M1 from influenza C virus (M1-C) has been shown to be the key component in inducing the formation of protrusions, called cord-like structures (CLS), emanating out of infected cells and in regulating their growth thus demonstrating a role for M1-C in membrane remodeling. We show that the N-terminal domain of M1-C adopts a similar fold as M1-A, despite the low sequence homology of both proteins, but coordinates two Mg2+ ions which increases the positive surface charge and may thus facilitate electrostatic interactions with negatively charged membranes. Full length M1-C adopts an elongated structure that tends to polymerize into ring-like or filamentous structures via lateral interactions of M1-C protomers. Our study thus confirms that M1-C assembly on membranes constitutes the driving force for influenza C virus bud formation.

We solved the crystal structure of C-terminally truncated M1-C, (NTD, residues 1–155) by single anomalous dispersion (SAD) techniques to a resolution of 1.5 Å. The structure is composed of a tandem repeat of two four-helical bundles (helices 1–4 and 6–9) that are connected by a long linker containing helix 5. Interactions between the two four helical bundles and with the linker are hydrophobic as in the case of M1-A structures28293139. The overall fold is similar to known M1-A NTD crystal structures28293139, albeit their low sequence homology. Major changes are observed for the position of helix 6, which moves approximately 10 Å outwards. A notable difference between the M1-A and M1-C structures is the unexpected coordination of 2 Mg2+ ions by helix 5 residues. The first Mg2+ ion is coordinated by Asn80, Asp130, Glu126 and three water molecules and the second Mg2+ ion interacts with Thr83, Glu123, Glu126 and three water molecules. Nevertheless the presence of Mg2+ may not have a structural role since circular dichroism showed no difference in melting temperature (TM = 62 °C) in the presence or absence of EDTA (ethylenediaminetetraacetic acid). However, the presence of the two Mg2+ ions changes the electrostatic potential of the M1-C surface. In the absence of Mg2+ this surface is substantially less positively charged, while in the presence of Mg2+, the basic charge distribution is similar to that of M1-A.

> MAHEILIAETEAFLKNVAPETRTAIISAITGGKSACKSAAKLIKNEHLPLMSGEATTMHIVMRCLYPEIKPWKKASDMLNKATSSLKKSEGRDIRKQMKAAGDFLGVESMMKMRAFRDDQIMEMVEEVYDHPDDYTPDIRIGTITAWLRCKNKKS methyl 1H-indole-4-carboxylate | C10 H9 N O2 | 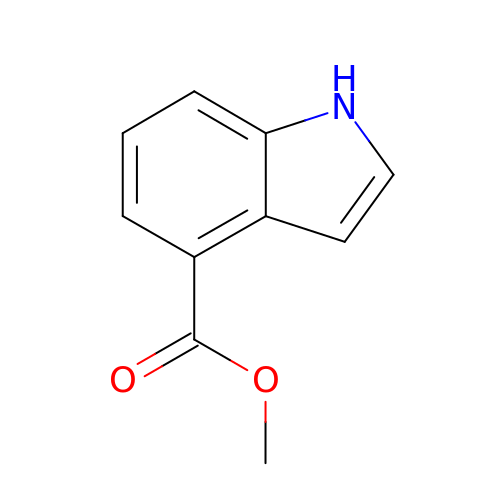WEAXQUBYRSEBJD-UHFFFAOYSA-N>GSMREESWEEHDTIQLTAQRKYLAEVQALETLLARELSVFLTEPGSKKTNIINRITGKTYALPSTELLRFYEHLEQCRKQGALMYFLERQGTYSGLMLDYDLKLNTNAAPSLESSVLSRLCHRIFVHIKNSSVLPEGSHKIHFFFTLKPEAVQGKYGFHVLIPGLKMAASTKKSIIASLQHDATVQKILHEQGVANPESCLDPHSASVPSLLYGSSKLNHRPYQLKTGFELVFDSSDPDYIPIHQIKNIESYNLVSELSLTNEQGSLVRPVYCAADIAAEKEEEIPADDHSLSILMLHDPEARYLHKILNLLPPEYYVEYPLWSNVVFALANTSANYRPLAEWFSQKCPEKWNTGGKEKLEKLWNDASRHTEKKITKRSIMYWAHKHAPQQYKEIVEQGYFSILAEYVYSYNGTLEHYMIAKVIYAMMGNKFVVDVDSNGKYVWFEFVLPGQPMNQGEIWKWRKEVNPDELHIYISENFSRVMDRITEHIKYHLSQPHETNILNYYKKLLKAFERSKSKIFNDSFKKGVIRQAEFLFRQRSFIQTLDTNPYLLGVGNGVLSIETIPAKLINHFHEHPIHQYTHICYEPFNPENPWTKLLLNALQDIIPELDARLWIMFYLSTAIFRGLKEALMLLWLGGGCNGKTFLMRLVAMVLGDHYASKLNISLLTSYRETAEKPNSAFMRLKGRGYGYFEETNKSEILNTSRLKEMVNPGDVTARELNQKQESFQMTATMVAASNYNFIIDTTDHGTWRRLRHYRSKVKFCHNPDPNNSYEKKEDPRFIHEYIMDPNCQNAFFSILVYFWEKLQKEYNGQIKKVFCPTIESETEAYRKSQDTLHRFITERVVESPSAETVYNLSEVVTAYAEWYNANINVKRHIALELSQELENSVLEKYLQWSPNKTRILKGCRILHKFETLQPGESYIGVSSTGTLLNTPICEPKNKWWEWSPNPSAPPEKEASAPTP[6x]

Here, we report the structural and biochemical studies of the highly conserved C962R protein of ASFV, showing that C962R is a multidomain protein. The N-terminal AEP domain is responsible for the DNA polymerization activity, whereas the DNA unwinding activity is catalyzed by the central SF3 helicase domain. The middle PriCT2 and D5_N domains and the C-terminal Tail domain all contribute to the DNA unwinding activity of C962R. C962R preferentially works on forked DNA, and likely functions in Base-excision repair (BER) or other repair pathway in ASFV.

To reveal the detailed basis for DNA unwinding by C962R, we carried out cryo-EM study for C962R in the presence of both DNA and AMPPNP. Therefore, instead of regular dsDNAs or dsDNAs with 3′-overhang, ssDNA was directly utilized in the cryo-EM study of the C962R-DNA-AMPPNP complex. However, different from the apo-form C962R structure, the two C962R hexamers are tilted with respect to each other in the ternary complex structure. Since the tilting angle varies from one particle to another, we only modeled one C962R hexamer in the final structure. In the complex structure, six AMPPNP molecules were captured by the C962R hexamer. The α and β phosphate groups of AMPPNP form four H-bond interactions with the main chain atoms of the Walker A motif (Gly638-Phe644); the γ phosphate group interacts with the side chain of Lys642 and Asn737. The DNA is located in the central channel of the C962R hexamer. Although no stable interaction was observed for the nucleobases, the backbones of the DNA form extensive H-bond interactions with C962R, especially Arg717 and Asn720 of the helicase domains. The two loops are termed DNA-interacting loop (DIL) 1 and 2, respectively. Both DIL-1 and DIL-2 loops are well defined in the complex structures, whereas they are completely disordered in the apo structure. The SF3 helicase domains are symmetrically arranged in the apo C962R structure, whereas they adopt an asymmetric conformation in the complex structure.> GSHMPPPDPAAMGTWKFFRASVDGRPVFKKEFDKLPDQARAALIVLMQRY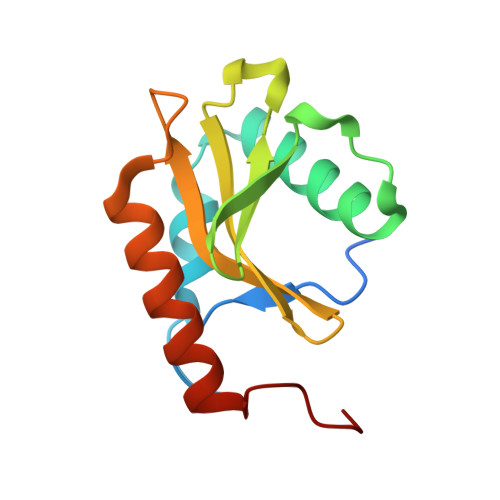LVGDLAAGSIKPIRGDILELRWHEANNHFRVLFFRWGQHPVALTAFYANQQKTPKTKIETALDRQKIWKRAFGDTPPILE>VCSCRLVFC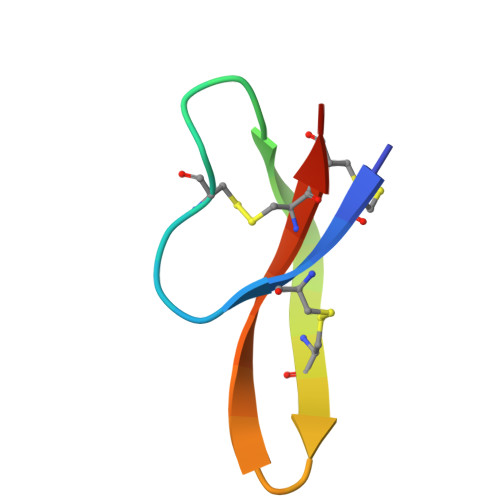RRTELRVGNCLIGGVSFTYCCTRV[4x]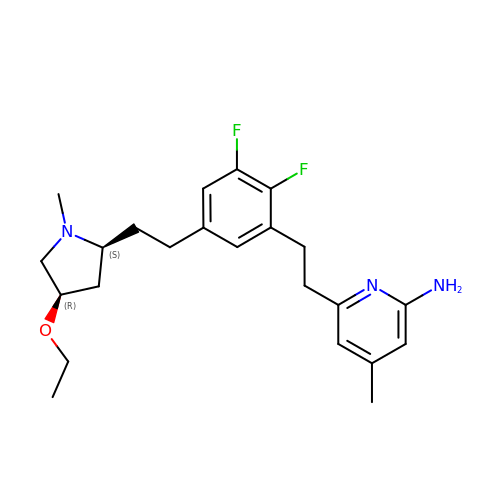6-[2-(5-{2-[(2S,4R)-4-ethoxy-1-methylpyrrolidin-2-yl]ethyl}-2,3-difluorophenyl)ethyl]-4-methylpyridin-2-amine | C23 H31 F2 N3 O | JJRCJHDDDMVMGM-VQTJNVASSA-N>GSHMSNTQTVLPFTGLNTPNGVAVDSAGTVYVTDHGNNRVVKLAAGSNTQTVLPFTGLNTPNGVAVDSAGTVYVTDHGNNRVVKLAAGSNTQTVLPFTGLNTPNGVAVDSAGTVYVTDHGNNRVVKLAAG[2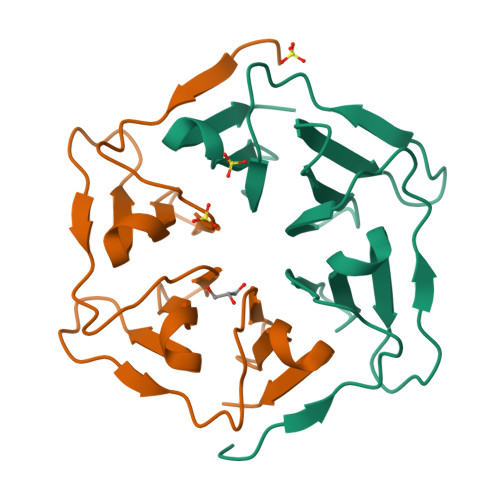x]> SHMQTPQALKIIVPYPAGGTADILPRVVAEKLRAQFPAGVLIDNRT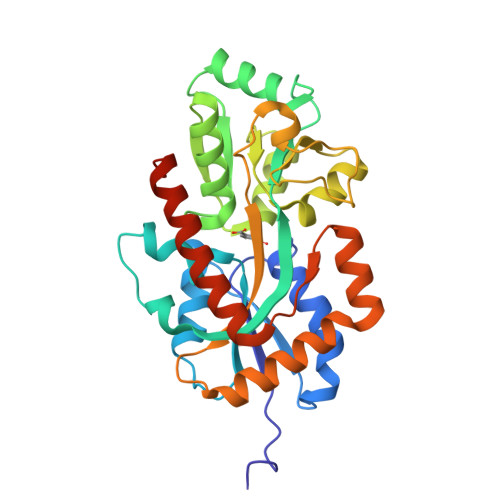GAGGNIGAEAVFRAEPDGNTLLASPPGPIAINHHLYRKMAFDPSKWEPVTVLATVPNVLVVNPRLPVKNVQEFIAYAKANPGKVTYGSQGNGTTSHLTASLFMQLTGTEMVHVPYKGTAPALVDLVGGQIDVFFDNISSSLPFHQAGKLRILGVADEQRSAALPEVPTFAEQGLPSMNAVTWFAVVAPPGTPAAKVAALQKSFAGALTQPEVQQKFAEQGAEPRGWDPARTGQFIRAESAKWDRVIRSANVRLDLEHHHHHH(2S)-2-hydroxy-3-(4-hydroxyphenyl)propanoic 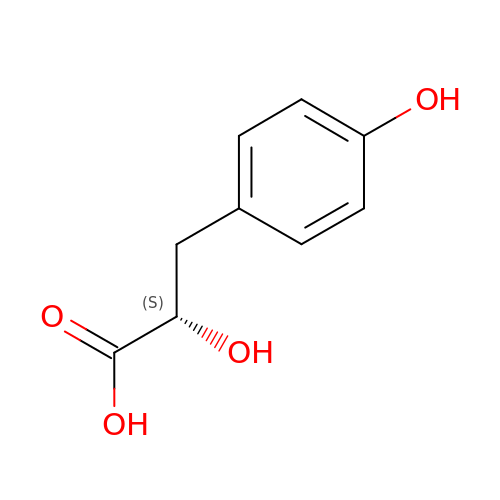acid | C9 H10 O4 | JVGVDSSUAVXRDY-QMMMGPOBSA-N>[24x]PKPYVAINMAELKNEPKTFEMFASVGPKVCMVTARHPGFVGFQNHIQIGILPFGNRYGGAKMDMTKESSTVRVLQYTFWKDWKDHEEMHRQNWSYLFRLCYSCASQMIWGPWEPIYEIIYANMPINTEMTDFTAVVGKKFAEGKPLDIPVISQPYGKRVVAFAEHSVIPGKEKQFEDAIVRTLEMLKKAPGFLGAMVLKEIGVSGIGSMQFGAKGFHQVLENPGSLEPDPNNVMYSVPEAKNTPQQYIVHVEWANTDALMFGMGRVLLYPELRQVHDEVLDTLVYGPYIRILNPMMEGTFWREYLNE

In this study, we present the cryo-EM structures of two thermostable multimeric enzymes that have different point-symmetry groups; namely SOR from Acidianus ambivalens and LS from Aquifex aeolicus. The reported cryo-EM structures of the two enzymes including their active sites correlate very well with the x-ray crystal structures. Due to their thermostability and relatively easy purification scheme, both SOR and LS can serve as a model for the catalytic and structural characterization of biocatalysts as well as a benchmark for cryo-EM sample preparation, optimization of the acquisition parameters and 3D reconstruction.

First, we determined the structure of the Sulfur Oxygenase Reductase (SOR) enzyme that catalyzes both the oxygenation and disproportionation of elemental sulfur in Archea and is composed of 24 homomeric units each of MW ≃ 35 kDa arranged in octahedral symmetry. The resolution of the final cryo-EM map was 2.78 Å according to the estimation from the Fourier shell correlation (FSC) at the 0.143 cut-off criterion. The average root mean square deviation (RMSD) between the cryoEM and x-ray crystal structures of SOR is 0.575 Å for the 307 Cα atoms. The core structure of the monomer is composed of eight β-strands surrounded by nine α-helices. The catalytic active site in each of the 24 monomeric subunits contains a mononuclear non-heme iron site, where the Fe3+ ion is responsible for the positive charge of the inner surface of the hollow cavity in SOR. The density of the side chains of H86, H90 and E114 surrounding the iron center, and that of two water molecules ligated to the Fe3+ ion are distinguishable in our cryo-EM map. Besides these three residues, there are three conserved cysteines; pursulfurated cysteine 31 (CSS31), C101 and C104 that are present in the active site and complete the hexa-coordination of the Fe3+ ion. The extra density in the cryo-EM map results from CSS31 existing in two rotamer conformations with equal occupancies. The characteristic feature for SOR is the presence of chimney-like protrusions at the 4-fold symmetry axes. These tetramer channel structures formed by the side chain of residues at each of four adjacent subunits are proposed to allow the sulfur substrates to access the inside of the hollow sphere cavity of SOR, where catalysis can take place secluded from the cytoplasmic environment. The exit routes of the polar products such as HSO3−, HS− and S2O32− are proposed to be the hydrophilic trimer channels formed by three subunits positioned along a 3-fold symmetry axis.> MNAPTTAAAGAAPGRQVKDSELLARLADPAARGDFPPGCRAHVRIDISIRAYWHTLFDICPGLLDIADPDGMAIFAPFMDWARRENLTMGWSFYIWVGRWLAQSPWRERLDEELTQALLSASAARWAVLDRSADVGVVLGRRGSDDWIIGWKPN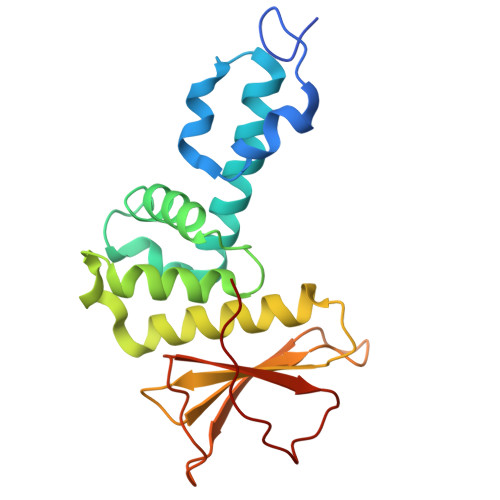TLAAGRRVELVSLDGQLPRPAEDVGVFHLAGYELDSFPGWLALPR N-{4-[3-(6-methoxypyridin-3-yl)-1H-pyrrolo[3,2-b]pyridin-2-yl]pyridin-2-yl}acetamide 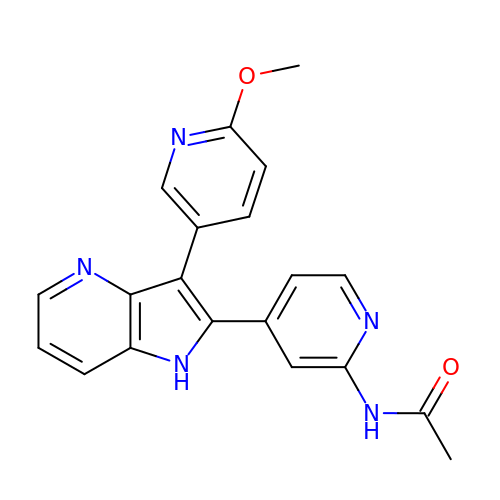| C20 H17 N5 O2 | XODSKPZUYKGNMW-UHFFFAOYSA-N>GSMTGASTTTATMRQRWQAVMMNNYGTPPIALASGDGAVVTDVDGRTYIDLLGGIAVNVLGHRHPAVIEAVTRQMSTLGHTSNLYATEPGIALAEELVALLGADQRTRVFFCNSGAEANEAAFKLSRLTGRTKLVAAHDAFHGRTMGSLALTGQPAKQTPFAPLPGDVTHVGYGDVDALAAAVDDHTAAVFLEPIMGESGVVVPPAGYLAAARDITARRGALLVLDEVQTGMGRTGAFFAHQHDGITPDVVTLAKGLGGGLPIGACLAVGPAAELLTPGLHGSTFGGNPVCAAAALAVLRVLASDGLVRRAEVLGKSLRHGIEALGHPLIDHVRGRGLLLGIALTAPHAKDAEATARDAGYLVNAAAPDVIRLAPPLIIAEAQLDGFVAALPAILDRAVGAP[4x]

The L-arginine biosynthesis pathway consists of eight enzymes that catalyse the conversion of L-glutamate to L-arginine, appears to be attractive target for anti-Tuberculosis (TB) drug discovery. The arginine biosynthesis pathway consists of eight different enzymes ([Fig fig1]) all considered to be essential for *M. tuberculosis* growth *in vitro*. In this work, the ligandability of four enzymes of the pathway ArgB, ArgC, ArgD and ArgF is explored using a fragment-based approach. In conclusion, using a fragment-based approach, we have discovered inhibitors that bind to novel sites in ArgB and ArgF and to the active sites of ArgC and ArgD, which in case of ArgB show on target activity against *M. tuberculosis*.

The first crystal structure of the ArgD holoenzyme from *M. tuberculosis* obtained ([Fig fig3]) showed that the protomer has three domains: the smaller N-terminal segment (residues 7 to 74), the relatively larger C-terminal domain (residues 286 to 396), and the central PLP-binding domain (residues 85 to 273), which is also the largest and has a Rossmann-like overall fold ([Fig fig3]). The prosthetic group PLP is covalently linked to Lys253 via an aldimine linkage. (a) X-ray crystal structure of *M. tuberculosis* ArgD showing the dimer. ArgD contains the prosthetic group PLP that does not leave the active site of the enzyme. Therefore, all the PLP sites must remain occupied during screening experiments to represent the native state of the target. While ArgB and ArgC do not have a human orthologue, ArgD and ArgF do and the *M. tuberculosis* enzymes have identities of 36 and 41% with the human orthologues, respectively. For ArgD selectivity might be more difficult to achieve since many of the active site residues are conserved in comparison with the human cytoplasmic and mitochondrial enzymes.>[12x]MGKVYKKVELVGTSEEGLEAAIQAALARARKTLRHLDFFEVKEIRGTIG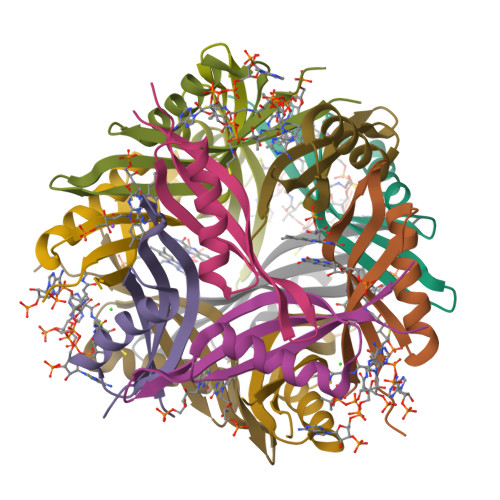EAGVKEYQVVLEVGFRLEET> MRGSHHHHHHGSMPFEIVFEGAKEFAQLIETASRLIDEAAFKVTEEGISMRAMDPSRVVLIDLNLPASIFSKYEVDGEETIGVNMDHLKKVLKRGKAKETLILRKGEENFLEISLQGTATRTFKLPLIDVEEIEVDLPELPFTAKVVILGDVIKEAVKDASLVSDSMKFIAKENEFTMRAEGETQEVEVKLTLEDEGL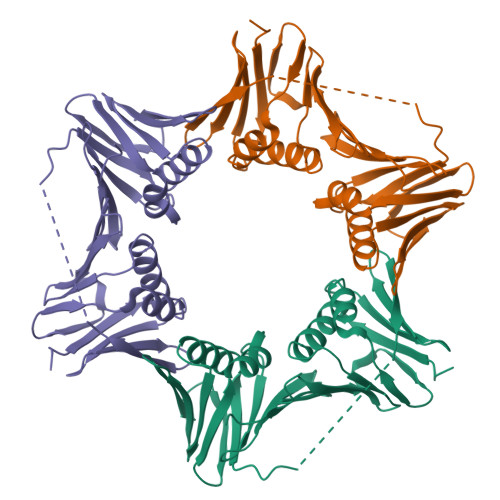LDIEVQEETKSAYGISYLSDMVKGLGKADEVTIKFGNEMPMQMEYYIRDEGRLIFLLAPRVEE> GFPWV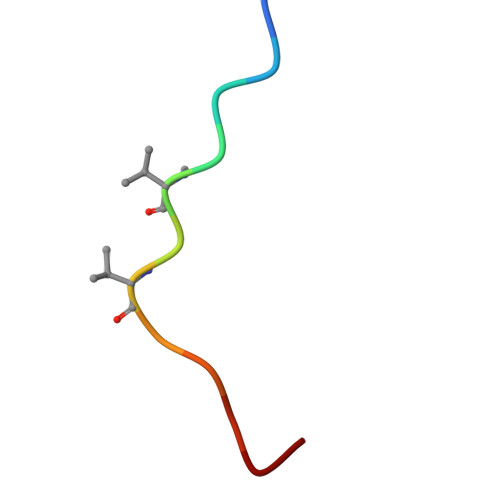IVVGVPG> MNLKDSIGLRIKTERERQQMSREVLCLDGAELTVRQLIRIEKGESLPSLDRLSYIAKRLGKSMTELLDQDNITIPDEYYEMKNRLIKFPTYRNPDRIKSKLTLIEEVYEKFFDILPEEELLTLDILENILSFTSWEESPKVEEIYEDLFEQVKRKRKFSTNDLLVIDYYFFHLYGRKQYDKKLFERIIKRVLNQEIWTDDVYNIVLFNDLMAIAALKIFHNSFSDFLTVVDKALAVIEKSQLYSYKPSVFVLKAKYELLHKENKKEAAENYDKAIVFASVLEDSVLEESIKAGKLADGLGAGWSHPQFEK

Here, we elucidate the structure-function relationship of the transcription factor ComR, a new member of the RNPP family, which positively controls competence for natural DNA transformation in streptococci. ComR is directly activated by the binding of its associated pheromone XIP, the mature form of the comX/sigX-inducing-peptide ComS. XIP-binding induces release of the sequestered HTH domain and ComR dimerization to allow DNA binding. Each TPR domain is composed of 11 α-helices forming 5 TPR motifs followed by an additional C-terminal α-helix α16 called CAP.

The crystal structure of the apo form of ComR from S. thermophilus has been determined at a resolution of 1.95 Å in the space group C 2 2 2 with 1 molecule per asymmetric unit. Assembly analysis of the crystal contacts using PDBePISA suggested that apo ComR is a monomer. Size Exclusion Chromatography combined to Multi Angle Laser Light Scattering (SEC-MALLS) analysis clearly established that apo ComR is a monomer in solution, with a measured molecular weight of 41 kDa for a calculated value of 36.5 kDa. In the absence of peptide, the HTH domain is sequestered by the TPR domain of the ComR monomer, generating a new interface of 874.9 Å2. Interestingly, this interface involves the HTH residues R35, R39 and R51, which have been shown to be directly implicated in DNA-binding. In the apo form of the protein, they form salt bridges with TPR-2 residues: R35 with E146 and D147, R39 with E117, and R51 with E118. The residue pair E117-E118, which belongs to the strongly conserved L115PEEE119 motif located in loop α7-α8 between TPR-1 and TPR-2, thus plays an important role in stabilizing the inactive apo form of the protein. Superimposition of the apo and bound forms of the ComR TPR domain (rmsd of 2.4 Å over 212 aligned Cα atoms) showed that the main difference concerns helix α9, which was broken in the dimeric complex and forms a more canonical TPR-2 motif in the apo structure. Interestingly, crystal contacts generate a dimerization interface similar to the dimeric bound form of the protein, with a conserved K246-E282 salt bridge. However, the small overall interface (537.9 Å2) and the poor calculated solvation free energy gain (ΔiG of -1.9 kcal.mol-1) characterizing this contact in the apo structure suggest that the monomer-dimer equilibrium is shifted toward the monomeric form in the absence of peptide and that the dimer would not be stable in the absence of crystal packing forces.>[6x]MAKEKARYFTFLLYPESIP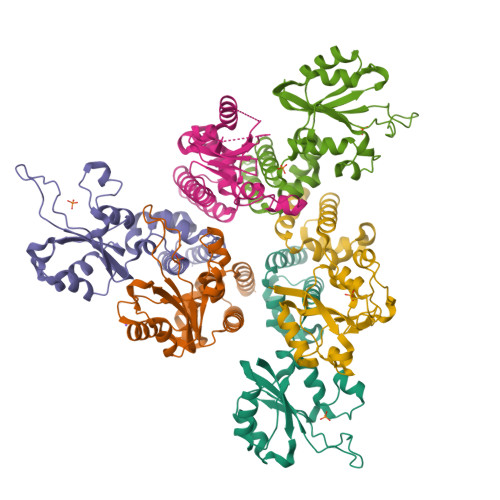SDWELKLETLGVPMAISPLHDKDKSSIKGQKYKKAHYHVLYIAKNPVTADSVRKKIKLLLGEKSLAMVQVVLNVENMYLYLTHESKDAIAKKKHVYDKADIKLINNFDIDRYVTLDVEEKTELFNVVVSLIRAYTLQNIFDLYDFIDENGETYGLTINLVNEVIAGKTGFMKLLFDGAYQRSKRGTKNEER> GVEITEGVTVTAKGNTEGNTADLAIDGDLSTYWESSNDYKWIEVDLGGIYELSKIEIFNKDEAVYKYNIYASEDGENFNKIAYKNNDNVSDSNGNMHTIDNVRAGKIRIDVVQNSNSDRVNIAEINVFGKNTGESLPEVKKIATSNFSETPWATEYEKFNSDSAYANEKTLNEIKNLVGRVIGREFKDKFIFEIRDQLNGNDVFEVSDSGDGKVLIKGNNGVSLASGFNYYLKNYCNVSYNPIMGSNLKMPETMPSVGERVVIDTPYEHRYALNFCTYSYTMSFWDWDQYEEFLDWCAMNGVNLVLDIIGQEEVLRRTLNEFGYSDEEVKEFISGPAYFAWFYMQNMTGFGGPLPNDWFEQRAEL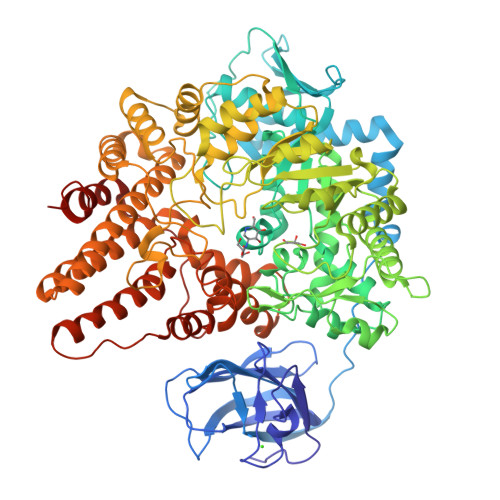GRKMHDRMQSFGINPVLQGYSGMVPRDFKEKNQEAQTISQGGWCGFDRPDMLKTYVNEGEADYFQKVADVFYEKQKEVFGDVTNFYGVDPFHEGGNTGDLDNGKIYEIIQNKMIEHDNDAVWVIQNWQGNPSNNKLEGLTKKDQAMVLDLFSEVSPDWNRLEERDLPWIWNMLHNFGGRMGMDAAPEKLATEIPKALANSEHMVGIGITPEAINTNPLAYELLFDMAWTRDQINFRTWTEDYIERRYGKTNKEILEAWNIILDTAYKKRNDYYQGAAESIINARPGFGIKSASTWGHSKIVYDKSEFEKAIEIFAKNYDEFKDSDAFLYDFADILKQLLANSAQEYYEVMCNAYNNGNGEKFKFVSGKFLELIKLQERVLSTRPEFLIGNWIEDARTMLKDSDDWTKDLFEFNARALVTTWGSRNNADGGGLKDYSNRQWSGLTEDYYYARWEKWINGLQAELDGGAKAPNIDWFKMEYDWVNKKSDTDKLYPTEASNENLGELAKIAMESYSVTNMDKILGENES> MGHHHH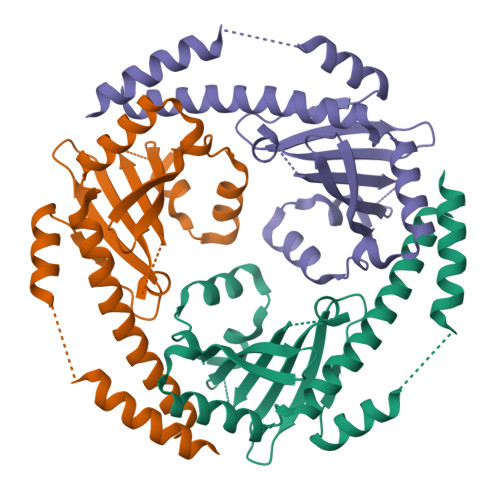HHQETQRVGDILQSELKIEKETLPESTSLDSFNDFLNKYKFSLVETPGKNEAEIVRRTESGETVHVFFDVAQIANLPYNNAMDENTEQNEDGINEDDFDALSDNFANVNVVISKESASEPAVSFELLMNLQEGSFYVDSATPYPSVDAALNQSAEAEITRELVYHGPPFSNLDEELQESLEAYLESRGVNEELASFISAYSEFKENNEYISWLEKMKKFFH>[4x]ADTIVAVELDTYPNTDIGDPNYQHIGINIKSIRSKATTRWNVQDGKVGTAHISYNSVAKRLSAIVSYPGGSSATVSYDVDLNNI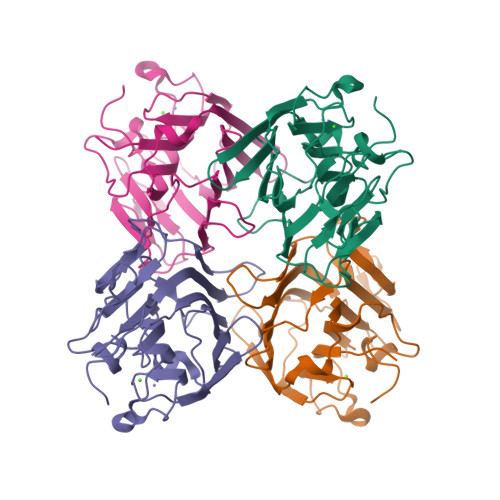LPEWVRVGLSASTGLYKETNTILSWSFTSKLKTNSTADAQSLHFTFNQFSQNPKDLILQGDASTDSDGNLQLTRVSNGSPQSNSVGRALYYAPVHVWDKSAVVASFDATFTFLIKSTDSDIADGIAFFIANTDSSIPHGSGGRLLGLFPDAN2-FORMYLPHENYL DIHYDROGEN PHOSPHATE | C7 H7 O5 P | 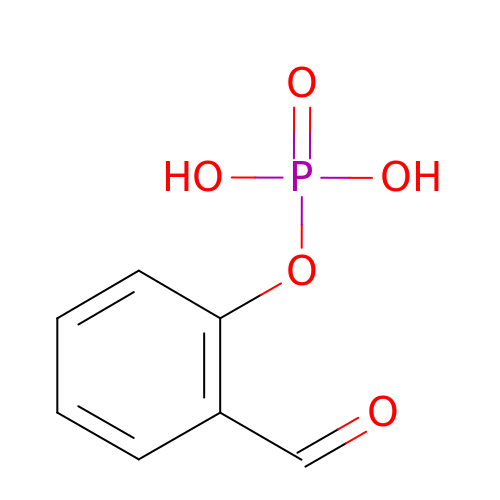BYNSFVCWJXZPOW-UHFFFAOYSA-N>APVRSLNCTL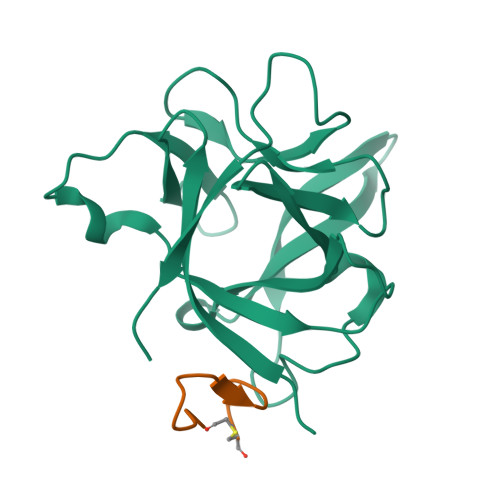RDSQQKSLVMSGPYELKALHLQGQDMEQQVVFSMSFVQGEESNDKIPVALGLKEKNLYLSCVLKDDKPTLQLESVDPKNYPKKKMEKRFVFNKIEINNKLEFESAQFPNWYISTSQAENMPVFLGGTKGGQDITDFTMQFVSS[2x];>[2x]FWDSWGYWYGPWDCGKX>[2x]GPGGSPYLITGIPKDPKHPLPIRKDIDDWYLEQTSAGSNRIQLTLFVEALTVIQNRPLNDQLSYFRLAGIHGAPWTEWDGVPGGQKDSKGNP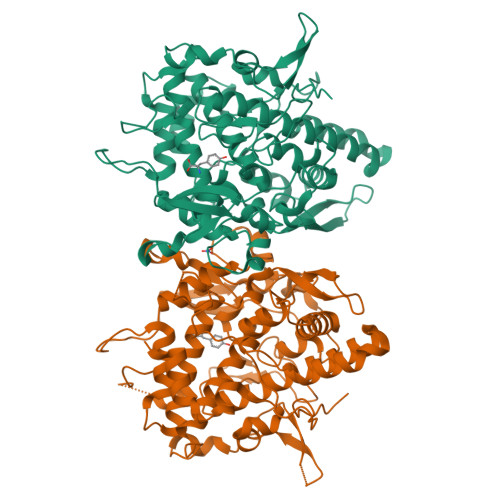TGFAVHNNYTFPTWHRVYVTLYEQVIYEAMLDFIKQNVPQNGKADWENEAKQWRLPYWDFARFARHGHDNTQGDELRLPILVTMPMVKVLVPGQPGKQLSKPNPLYRFQMQTLMGTLERPYAITSQKTEEHGWSFDLPFDKCQSTTKYGLLENYNADVWADGGQNWLRANLALNEHPWYQNLDGWDSVPTLQDMTFRLLTTGGLNWGEFSSTRYDDKKEETQPKNNEQAPKNWMNLEAIHNNVHNWVGGFMFSRPGRHDLKLWGAGHMSSVPVAAYDPIFWLHHCNIDRLTAIWQTVNSGSWFNDDKSKVSKDDDLRPFHRFCEKTRKVVFFRSDDVKDWRSLNYDYAITKDASRIRKEISDLYGQRTK>HFVQQKVKVFRAADPLVGVFLWGVAHSINELSQVPPPVMLLPDDFKASSKIKVNNHLFHRENLPSHFKFKEYCPQVFRNLRDRFGIDDQDYLVSLTRNPPSESEGSDGRFLISYDRTLVIKEVSSEDIADMHSNLSNYHQYIVKCHGNTLLPQFLGMYRVSVDNEDSYMLVMRNMFSHRLPVHRKYDLKGSLVSREASDKEKVKELPTLKDMDFLNKNQKVYIGEEEKKIFLEKLKRDVEFLVQLKIMDYSLLLGIHDIIRGSEP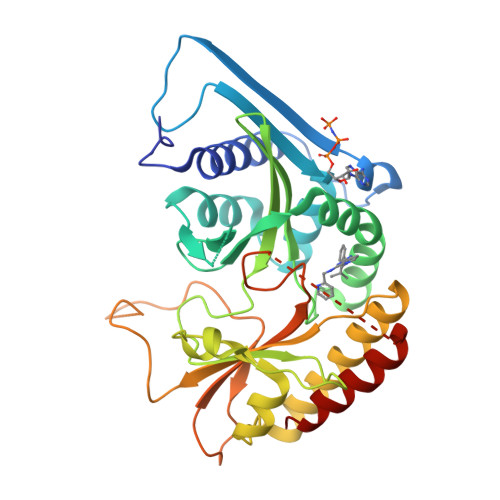EEELGPGEFESFIDVYAIRSAEGAPQKEVYFMGLIDILTQYDAKKKAAHAAKTVKHGAGAEISTVHPEQYAKRFLDFITNIFA[2x]> SGSGSGSGSGSEFNATQINEELYRLLEDTEILNQEITEGLLKGFEVPDAGVAIQLSKRDVVYPARILIIVLSEMWRFGLTKQSESFLAQVLTTIQKVVTQLKGNDLIPSGVFWLANVRELYSFVVFALNSILTEETFKNGMTDEEYKEYVSLVTELKDDFEALSYNIYNI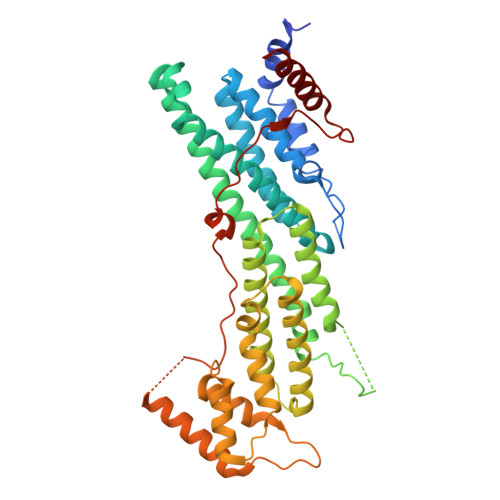WLKKLQKQLQKKAINAVVISESLPGFSAGETSGANTEEYTMDDILTFFNSIYWCMKSFHIENEVFHAVVTTLLNYVDAICFNELIMKRNFLSWKRGLQLNYNVTRLEEWCKTHGLTDGTECLQHLIQTAKLLQVRKYTIEDIDILRGICYSLTPAQLQKLISQYQVADYESPIPQEILRYVADIVKKEAALSSSGNDSKGHEHSSSIFITPETGPFTDPFSLIKTRKFDQVEAYIPAWLSLPSTKRIVDLVAQQVVQDGH3-[(3R)-3-(imidazo[4,5-d]pyrrolo[2,3-b]pyridin-1(6H)-yl)piperidin-1-yl]-3-oxopropanenitrile | C16 H16 N6 O | 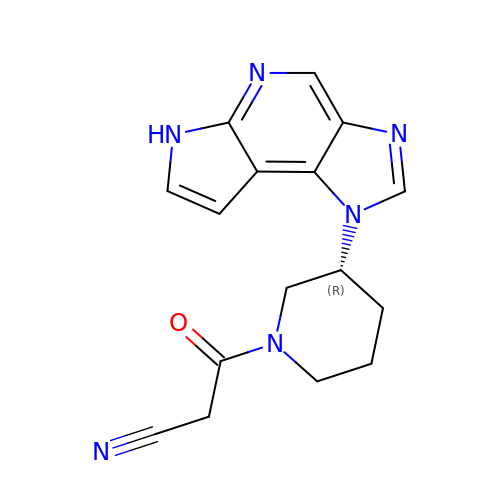XTKGOBBIBUQFHY-LLVKDONJSA-N>GPPTSDDIFEREYKYGAHNYHPLPVALERGKGIYLWDVEGRKYFDFLSSYSAVNQGHCHPKIVNALKSQVDKLTLTSRAFYNNVLGEYEEYITKLFNYHKVLPMNTGVEAGETACKLARKWGYTVKGIQKYKAKIVFAAGNFWGRTLSAISSSTDPTSYDGFGPFMPGFDIIPYNDLPALERALQDPNVAAFMVEPIQGEAGVVVPDPGYLMGVRELCTRHQVLFIADEIQTGLARTGRWLAVDYENVRPDIVLLGKALSGGLYPVSAVLCDDDIMLTIKPGEHGSTYGGNPLGCRVAIAALEVLEEENLAENADKLGIILRNELMKLPSDVVTAVRGKGLLNAIVIKETKDWDAWKVCLRLR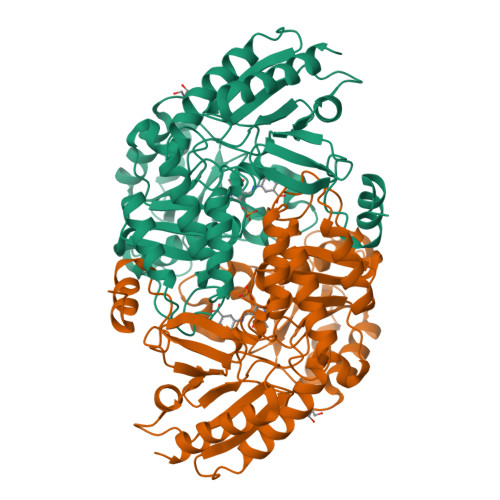DNGLLAKPTHGDIIRFAPPLVIKEDELRESIEIINKTILSF[3x]>[2x]MATVSRLRPYATTVFAEMSALATRIGAVNLGQGFPDEDGPPKMLQAAQDAIAGGVNQYPPGPGSAPLRRAIAAQRRRHFGVDYDPETEVLVTVGATEAIAAAVLGLVEPGSEVLLI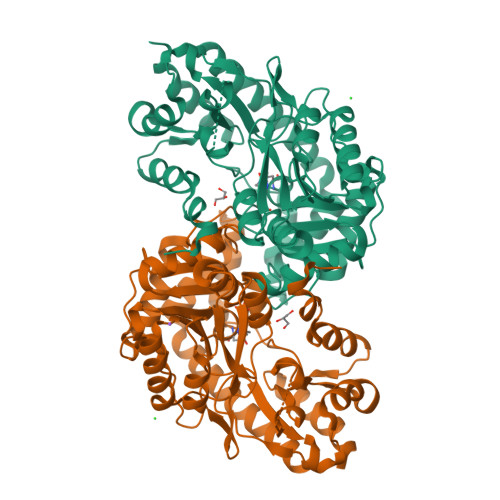EPFYDSYSPVVAMAGAHRVTVPLVPDGRGFALDADALRRAVTPRTRALIINSPHNPTGAVLSATELAAIAEIAVAANLVVITDEVYEHLVFDHARHLPLAGFDGMAERTITISSAAKMFNCTGWKIGWACGPAELIAGVRAAKQYLSYVGGAPFQPAVALALDTEDAWVAALRNSLRARRDRLAAGLTEIGFAVHDSYGTYFLCADPRPLGYDDSTEFCAALPEKVGVAAIPMSAFCDPAAGQASQQADVWNHLVRFTFCKRDDTLDEAIRRLSVLAERPATGVPRGLEHHHHHH> GSVYPKELTQVFEHYINNNLFDIDSLVKFIEELGYNLEDLATLCLAHLLGYKKLEEPLKREDFLSTWFMQGCSTISDMQECIKTLDVKLHEDLQYFTQIYNYAFNLILDPN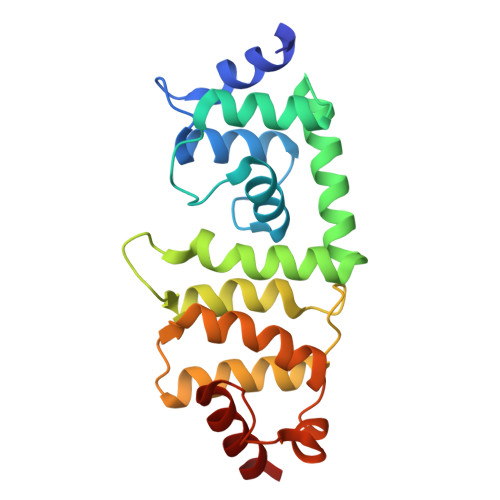RKDIDTDEGIQYWKLFFQPEYPVRMEPDLLEAWFRFLRDEGKTTISKDTWRMLLLFFKRYPTIQKIISDYDETAAWPFIIDEFYECLQDQQ> HEVVKFMDVYQRSYCHPIETLVDIFQEYPDEIEYIFKPSCVPLMRCGGCCNDEGLECVPTEESNITMQIMRIKPHQGQHIGEMSFLQHNKCECRPK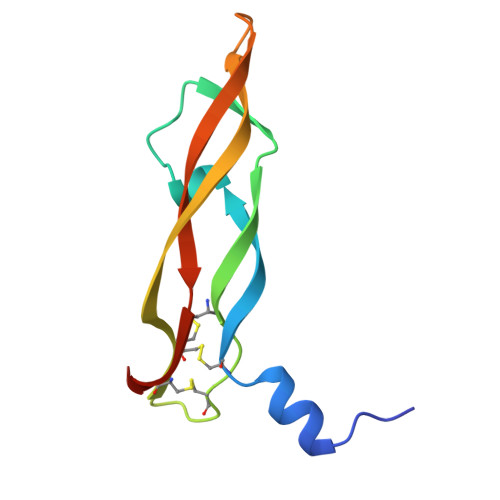KD>MGSHHHHHHSSGENLYFQGHMFKKLENLEKWEPPKDWMVIKTLDTHTAGEPLRIILSGFPEIPGKTILEKRRYLM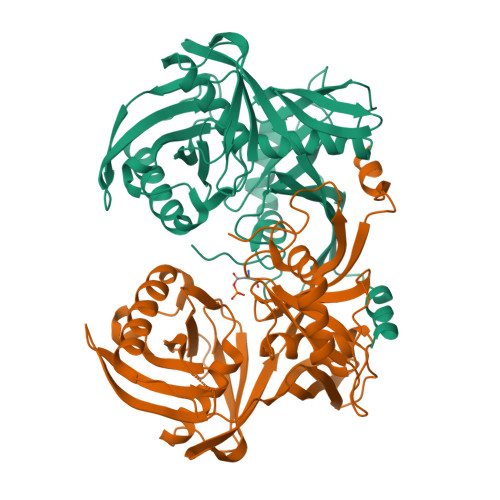ENLDHLRKALMWEPRGHADMYGAIITEPVSEEADFGVIFMHNEGYSTMCGHATIALGKVAVECGLVEAKEPITEIKMDSPAGLIKIYVKVRDGKVEKVYFHNVPSFVLFKDETINVPGIGEVKYDLAYGGAFYAFVNAEEIGLKCTPEYYRQLIDVGMKIKRAIMSEKEIRHPFEEDLSFLYGTIFIGEPEDENSHSRHVCIFADGEVDRSPTGTGVSARLAILYEKGEIDIGEEITIESIIGTKFTGKVVEETRYGLYRAIIPEVGGNAYIVAKNTFLIDPQDPLKYGFFLR[4x]> MAEDFVSENSNNKRAPYWTNTEKMEKRLHAVPAANTVKFRCPAGGNPMPTMRWLKNGKEFKQEHRIGGYKVRNQHWSLIMESVVPSDKGNYTC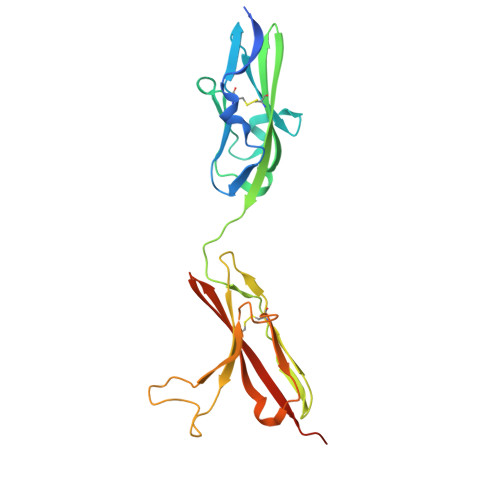VVENEYGSINHTYHLDVVERSRHRPILQAGLPANASTVVGGDVEFVCKVYSDAQPHIQWIKHVEKNGSKYGPDGLPYLKVLKHSGINSSNAEVLALFNVTEADAGEYICKVSNYIGQANQSAWLTVLPKQQAPGREKE~{N}-[[1-[(4-chlorophenyl)methyl]-1,2,3-triazol-4-yl]methyl]-2-hydrosulfonyl-2-methyl-propanamide 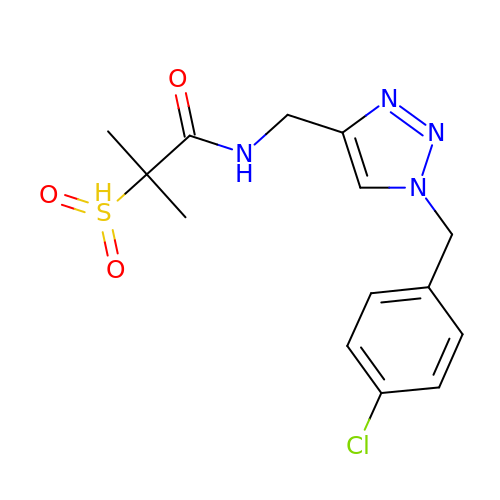| C14 H17 Cl N4 O3 S | WWIJWVXKLYGOJA-UHFFFAOYSA-N>[2x]MKDLVDTTEMYLRTIYELEEEGVTPLRARIA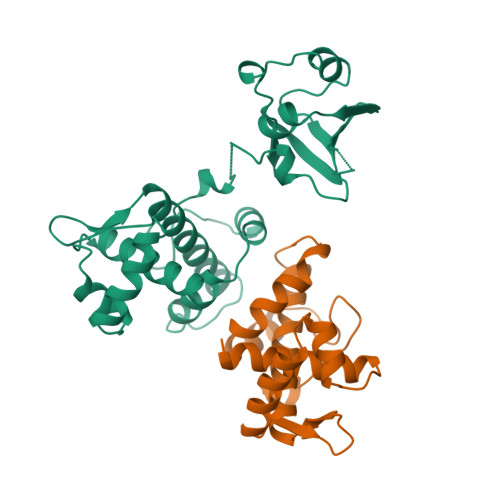ERLEQSGPTVSQTVARMERDGLVVVASDRSLQMTPTGRTLATAVMRKHRLAERLLTDIIGLDINKVHDEACRWEHVMSDEVERRLVKVLKDVSRSPFGNPIPGLDELGVGNSDAAAPGTRVIDAATSMPRKVRIVQINEIFQVETDQFTQLLDADIRVGSEVEIVDRDGHITLSHNGKDVELLDDLAHTIRIEEL> MLEQPYLDLAKKVLDEGHFKPDRTHTGTYSIFGHQMRFDLSKGFPLLTTKKVPFGLIKSELLWFLHGDTNIRFLLQHRNHIWDEWAFEKWVKSDEYHGPDMTDFGHRSQKDPEFAAVYHEEMAKFDDRVLHDDAFAAKYGDLGLVYG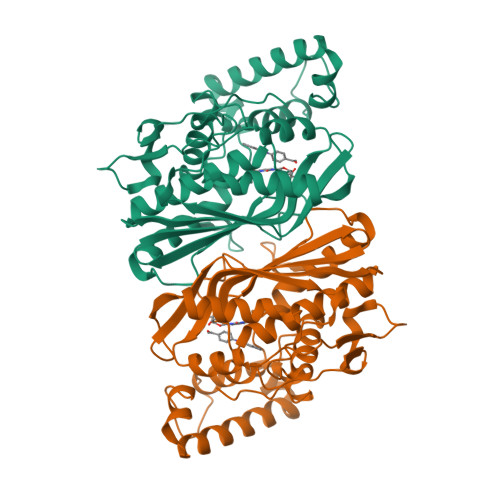SQWRAWHTSKGDTIDQLGDVIEQIKTHPYSRRLIVSAWNPEDVPTMALPPCHTLYQFYVNDGKLSLQLYQRSADIFLGVPFNIASYALLTHLVAHECGLEVGEFIHTFGDAHLYVNHLDQIKEQLSRTPRPAPTLQLNPDKHDIFDFDMKDIKLLNYDPYPAIKAPVAV> MQNVKGGYWFKDSGLALNNIDSTLFTHLFCAFADLNPQLNQLIISPENQDSFRQFTSTVQRKNPSVKTFLSIAGGRANSTAYGIMARQPNSRKSFIDSSI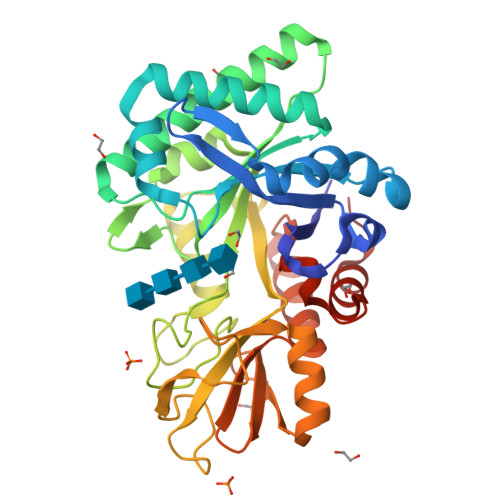RLARQLGFHGLDLDWQYPLSAADMTNLGTLLNEWRTAINTEARNSGRAALLLTAAVSNSPRVNGLNYPVESLARNLDWINLMAYDFYGPNWSPSQTNSHAQLFDPVNHVSGSDGINAWIQAGVPTKKLVLGIPFYGYAWRLVNANIHGLRAPAAGKSNVGAVDDGSMTYNRIRDYIVESRATTVYNATIVGDYCYSGSNWISYDDTQTVRNKVNYVKGRGLLGYFAWHVAGDQNWGLSRTASQTWGVSFQEMK>[2x]MKRSKRFAVLAQRPVNQDGLIGEWPEEGLIAMDSPFDPVSSVKVDNGLIVELDGKRRDQFDMIDRFIADYAINVERTEQAMRLEAVEIARMLVDIHVSREEIIAITTAITPAKAVEVMAQMNVVEMMMALQKMRARRTPSNQCHVTNLKDNPVQIAADAAEAGIRGFSEQETTVGIARYAPFNALALLVGSQCGRPGVLTQCSVEEATELELGMRGLTSYAETVSVYGTEAVFTDGDDTPWSKAFLASAYASRGLKMRYTSGTGSEALMGYSESKSMLYLESRCIFITKGAGVQGLQNGAVSCIGMTGAVPSGIRAVLAENLIASMLDLEVASANDQTFSHSDIRRTARTLMQMLPGTDFIFSGYSAVPNYDNMFAGSNFDAEDFDDYNILQRDLMVDGGLRPVTEAETIAIRQKAARAIQAVFRELGLPPIADEEVEAATYAHGSNEMP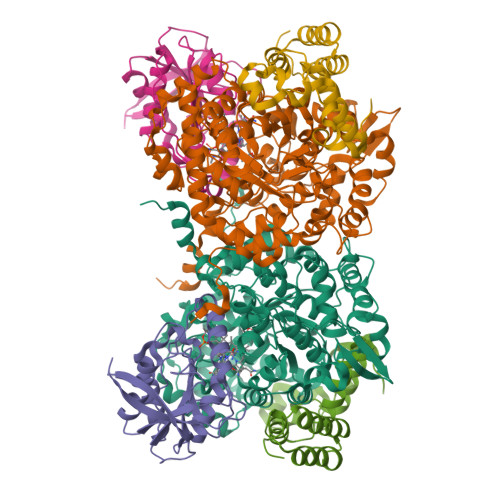PRNVVEDLSAVEEMMKRNITGLDIVGALSRSGFEDIASNILNMLRQRVTGDYLQTSAILDRQFEVVSAVNDINDYQGPGTGYRISAERWAEIKNIPGVVQPDTIE;>[2x]MQQTTQIQPSFTLKTREGGVASADERADEVVIGVGPAFDKHQHHTLIDMPHGAILKELIAGVEEEGLHARVVRILRTSDVSFMAWDAANLSGSGIGIGIQSKGTTVIHQRDLLPLSNLELFSQAPLLTLETYRQIGKNAARYARKESPSPVPVVNDQMVRPKFMAKAALFHIKETKHVVQDAEPVTLHIDLVRE;>MSEKTMRVQDYPLATRCPEHILTPTGKPLTDITLEKVLSGEVGPQDVRISRQTLEYQAQIAEQMQRHAVARNFRRAAELIAIPDERILAIYNALRPFRSSQAELLAIADELEHTWHATVNAAFVRESAEVYQQRHKLRKGS[2x]>SAVKAARYGKDNVRVYKVHKDEKTGVQTVYEMTVCVLLEGEIETSYTKADNSVIVATDSIKNTIYITAKQNPVTPPELFGSILGTHFIEKYNHIHAAHVNIVCHRWTRMDIDGKPHPHSFIRDSEEKRNVQVDVVEGKGIDIKSSLSGLTVLKSTNSQFWGFLRDEYTTLKETWDRILSTDVDATWQWKNFSGLQEVRSHVPKFDATWATAREVTLKTFAEDNSASVQATMYKM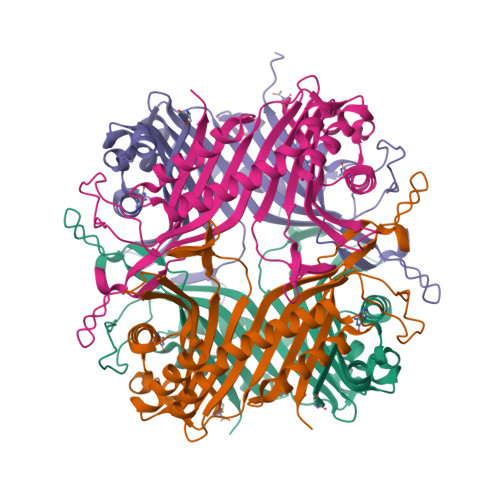AEQILARQQLIETVEYSLPNKHYFEIDLSWHKGLQNTGKNAEVFAPQSDPNGLIKCTVGRSSLKSKL[8x]>[2x]MLDGKQDNGNVDSVDIKQRTNGGGDEGDALGSNSSSQPNRVARMPVDRNAPYYNMNHKHRGMAIIFNHEHFDIHSLKSRTGTNVDSDNLSKVLKTLGFKVTVFPNLKSEEINKFIQQTAEMDHSDADCLLVAVLTAGELGMLYAKDTHYKPDNLWYYFTADKCPTLAGKPKLFFIQACQGDRLDGGITLSRTETDGSPSTSYRIPVHADFLIAFSTVPGYFSWRNTT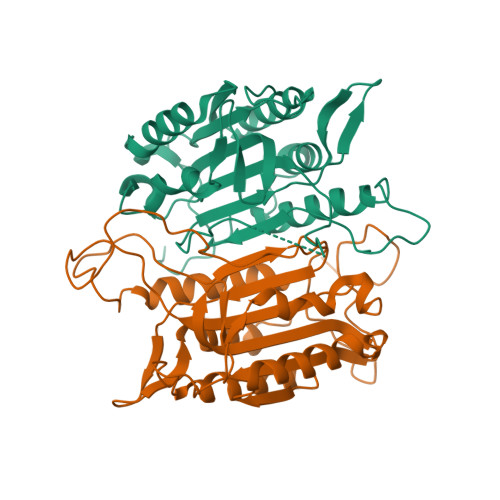RGSWFMQALCEELRYAGTERDILTLLTFVCQKVALDFESNAPDSAMMHQQKQVPCITSMLTRLLVFGKKQSHGGGLEHHHHHH FLAVIN-N7 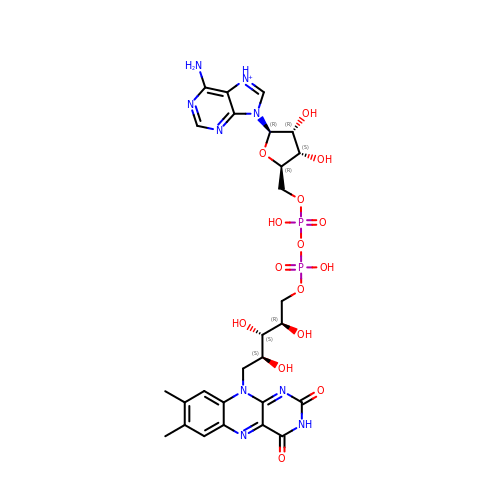PROTONATED-ADENINE DINUCLEOTIDE | C27 H34 N9 O15 P2 | VWWQXMAJTJZDQX-UYBVJOGSSA-O The RimK system allows for Pseudomonas spp. to adapt through post‐transcriptional regulation by altering the ribosomal subunit RpsF. RimK belongs to the ATP‐dependent carboxylate‐amine ligase superfamily of enzymes 13 , 24 which includes other members which can add amino acids to the C‐terminus of their target proteins. Each individual RimK unit has a classical ATP‐grasp fold with an elongated shape of approximately 60 x 35 x 30 Å. 25 The glutamate binding domain of each RimK subunit is linked to the ATP‐binding central domain by a flexible linker region, which is likely to allow the protein a range of motion to enable it to act like a classical “clam shaped” enzyme.

RimKPA was crystalized in the absence of its substrates; ATP, cdG, and glutamate whereas RimKPS was crystalized with both ATP and cdG present in the cryoprotectant. ADP and glutamate, of presumed cellular origin, were resolved in the RimKPA structure whereas ADP alone was resolved in the RimKPS structure. Within the RimKPS and RimKPA structures, the bound nucleotide was interpreted as ADP rather than ATP in the predicted ATP binding site, potentially due to a dephosphorylation event prior to crystallization. For RimKPS and RimKPA, the ADP molecule interacts with a core set of six side chains: K141, E178, I180, F210, S212, and N213. Within the upper loops, the β‐sheet of RimKPS is shorter than that of RimKPA, potentially allowing more flexibility in the loop. Although there is a high degree of sequence similarity between the active sites of the different RimK proteins, clear tertiary structure differences were present within their binding sites, with the RimKPS binding site appearing significantly more open than that of RimKEC. The residues H215, R216 and R211 are oriented in opposite directions in RimKEC and RimKPS, with all three pointing towards the active site in RimKEC, thus reducing the size of the active site cleft and encasing the ATP/ADP binding site. Previous work has shown that RimKPF and RimKPS are biochemically interchangeable, having similar ATPase activity levels and the ability to add an unlimited number of glutamate residues to RpsF, suggesting they have similar modes of action in vivo. Consequently, and as expected the addition of RimBPS stimulated RimKPS ATPase activity in a concentration dependent manner. The more closed active site conformation of RimKEC compared to RimKPA, itself presenting a more closed conformation than RimKPS, provides a possible explanation for the differences seen in V max and the enzymatic changes seen upon RimB binding.

>[16x]MKIAVLSRNPRLYSTRRLVEAGIERGHEMVVIDTLRAYMNIASHKPQIHYRGKPLEGFDAVIPRIGASVTFYGCAVLRQFEMMGVFPLNESVAIARSRDKLRSLQLLSRRGIGLPVTGFAHSPDDIPDLIQMVNGAPLVIKVLEGTQGIGVVLCETATAAESVIEAFMGLKQDIMVQEYIKEAGGADIRCFVVGDKVIASMKRQAKPGEFRSNLHRGGSASLIKITPEERMTALRAAKVMGLSVAGVDILRSNHGPLVMEVNSSPGLEGIEVTTSKDVAGMIIEYLEKNSGPHMTRTKGKGLEHHHHHH>[3x]AYRYRDIVVR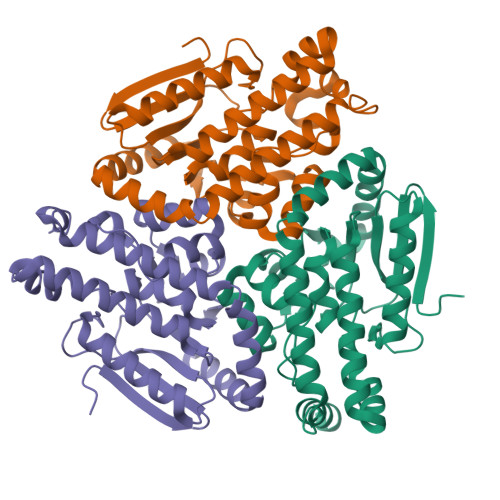KQDGFTHILLSTKSSENNSLNPEVMREVQSALSTAAADDSKLVLLSAVGSVFCCGLDFIYFIRRLTDDRKRESTKMAEAIRNFVNTFIQFKKPIIVAVNGPAIGLGASILPLCDVVWANEKAWFQTPYTTFGQSPDGCSTVMFPKIMGGASANEMLLSGRKLTAQEACGKGLVSQVFWPGTFTQEVMVRIKELASCNPVVLEESKALVRCNMKMELEQANERECEVLKKIWGSAQGMDSMLKYLQRKIDEF> SGRGKGGKGLG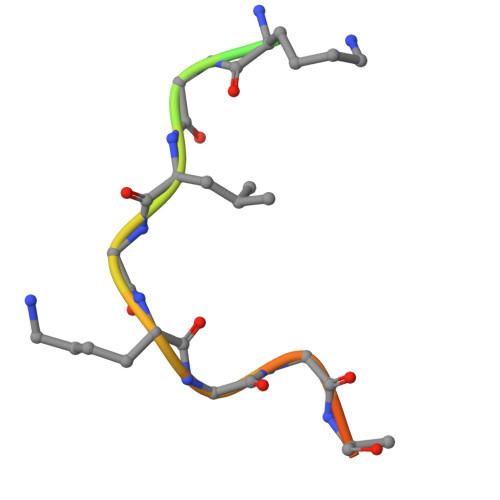KGGAKRHR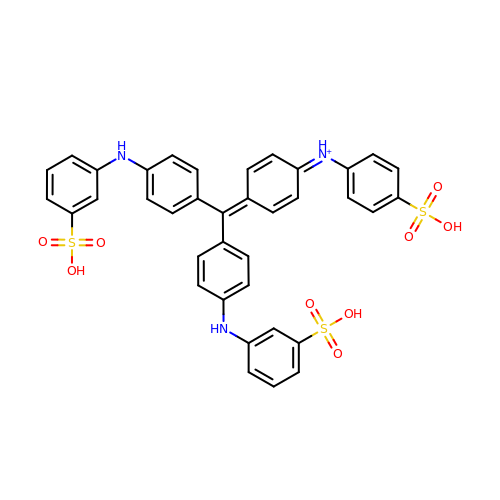N-[4-(BIS{4-[(3-SULFOPHENYL)AMINO]PHENYL}METHYLENE)CYCLOHEXA-2,5-DIEN-1-YLIDENE]-4-SULFOBENZENAMINIUM | C37 H30 N3 O9 S3 | QEJOESQJOWWNSS-UHFFFAOYSA-O(1R)-2-{[(S)-{[(2S)-2,3-dihydroxypropyl]oxy}(hydroxy)phosphoryl]oxy}-1-[(hexadecanoyloxy)methyl]ethyl (9Z)-octadec-9-enoate | C40 H77 O10 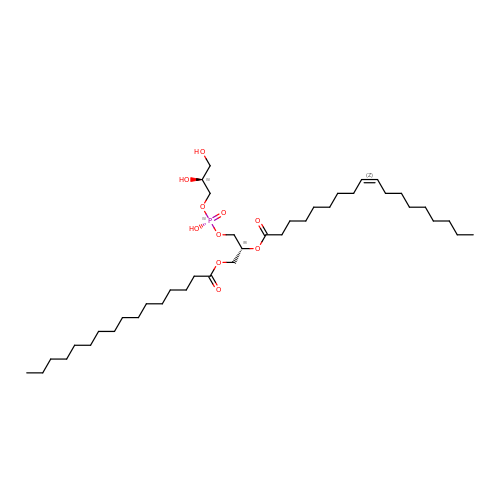P | PAZGBAOHGQRCBP-HGWHEPCSSA-N>MTEPLILQPAKPADACVIWLHGLGADRYDFMPVAEALQESLLTTRFVLPQAPTRPVTINGGYEMPSWYDIKAMSPARSISLEELEVSAKMVTDLIEAQKRTGIDASRIFLAGFSQ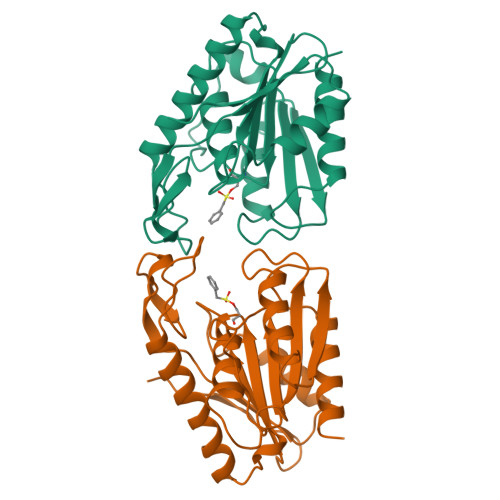GGAVVFHTAFINWQGPLGGVIALSTYAPTFGDELELSASQQRIPALCLHGQYDDVVQNAMGRSAFEHLKSRGVTVTWQEYPMGHEVLPQEIHDIGAWLAARLG[2x]> SSELFTLTYGALVTQLCKDY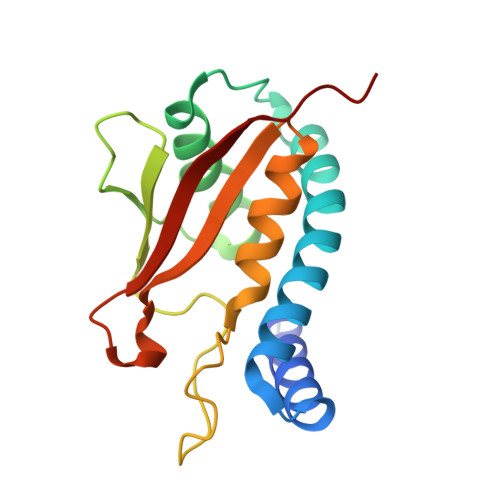ENDEDVNKQLDRMGYNIGVRLIEDFLARSNVGRCHDFRETADVIAKVAFKMYLGITPSITNWSPAGDEFSLILENNPLVDFVELPDNHSALIYSNLLCGVLRGALEMVQMAVEAKFVQDTLKGDGVTEIRMRFIRRIEDNL>MDPLYGYFAAVAGQDGQIDADELQRCLTQSGIAGGYKPFNLETCRLMVSMLDRDMSGTMGFNEFKELWAVLNGWRQHFISFDTDRSGTVDPQELQKALTTMGFRLSPQAVNSIAKRYSTNGKITF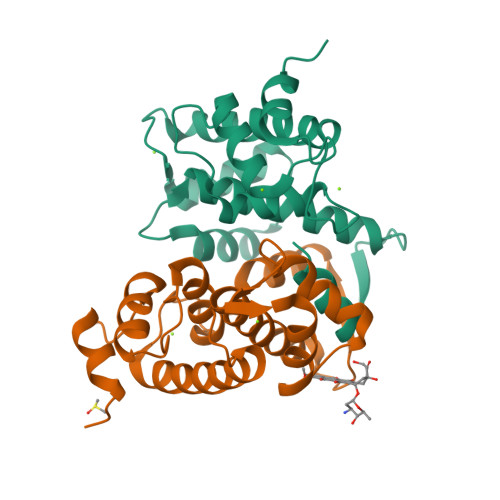DDYIACCVKLRALTDSFRRRDTAQQGVVNFPYDDFIQCVMSV[4x]>MG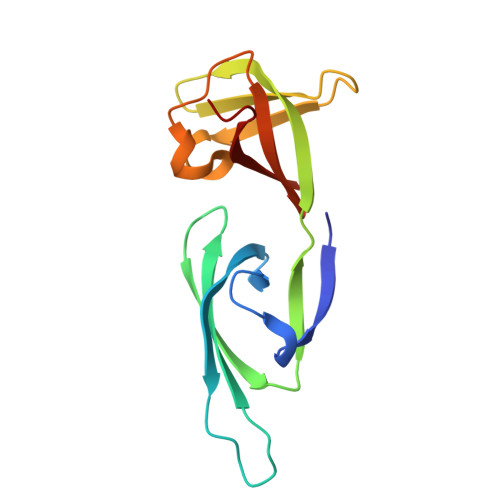DKTKVQVSKLKPGRYIIIDDEPCRIVNITVSSPGKHGSAKARIEAVGIFDGKVRSIVKPTSAEVDVPIIDKKTAQVIAITPDTVQIMDMETYETFEVPIDTGVADEIRDQLKEGINVEYWETLGRIKIMRIKGEGE[3x]> MGSSHHHHHHSSGPQQGLRQQQLVEVGNGYSQTSVNTTVFRNNSLVTQGDEQYISYYDGDGYLVLGKRKLDSDQWTLKRT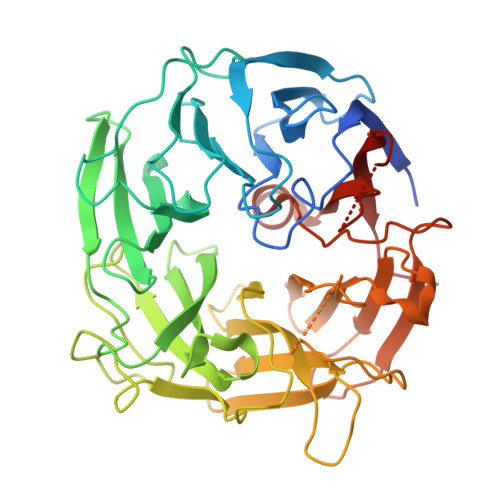QYKGNVKDAHNIISMMLDGEGYLHLSFDHHGHKLNYCRSTAPYTLELGDKEPMTGVDEGNVTYPEFYPLNGGDLLFVYRSGSSGRGNLVMNHYSVKEKKWNRVQDVLIDGEDQRNAYWQLYVDEQGTIHLSWVWRETWHVETNHDLCYARSYDNGVTWYKANGKKYDLPIRYNNAEYACRIPQNSELINQTSMSADASGNPYIATYWRDPDSEVPQYRIVWHDGQMWHNRQVSNRHTPFSLKGGGTKMIPIARPRIVVDGGEIFYIFRDEERGSRVSLAHAAAVGVGKWTFTDLTNFPVDAWEPSHDTELWKQKRRLHLFVQHTKQGDGERRVEFAPQPVYVLEVVKPKGD>SMALEIHMSDPMCLIENFNEQLKVNQEALEILSAITQPVVVVAIVGLYRTGKSYLMNKLAGKNKGFSVASTVQSHTKGIWIWCVPHPNWPNHTLVLLDTEGLGDVEKADNKNDIQIFALALLLSSTFVYNTVNKIDQGAIDLLHNVTELTDLLKARNSPDLDRVEDPADSASFFPDLVWTLRDFCLGLEIDGQLVTPDEYLENSLRPKQGSDQRVQNFNLPRLCIQKFFPKKKCFIFDLPAHQKKLAQLETLPDDELEPEFVQQVTEFCSYIFSHSMTKTLP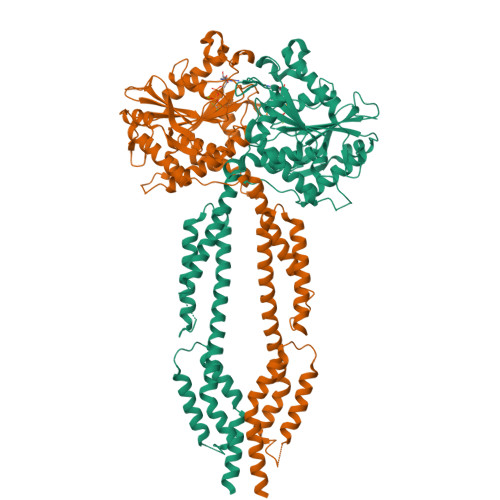GGIMVNGSRLKNLVLTYVNAISSGDLPCIENAVLALAQRENSAAVQKAIAHYDQQMGQKVQLPMETLQELLDLHATSEREAIEVFMKNSFKDVDQSFQKELETLLDAKQNDICKRNLEASSDYCSALLKDIFGPLEEAVKQGIYSKPGGHNLFIQKTEELKAKYYREPRKGIQAEEVLQKYLKSKESVSHAILQTDQALTETEKK[2x]(4S,5S)-4,5-BIS(MERCAPTOMETHYL)-1,3-DIOXOLAN-2-OL 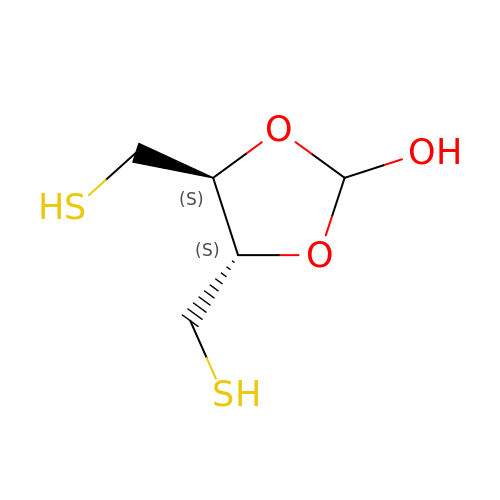| C5 H10 O3 S2 | URSOFHABYVLXDS-QWWZWVQMSA-N> MRRGALPQAPLERTRDFKGSAIRLARRLLPQRALTLAVILLGVGGIAIGVIGPRILGHATDLLFNGVIGRELPAGLTKEQAVEAARARGDGTFADLLSGMDIVPGQGVDFGAVGRTLALALGLYLVAALLVWVQARLLNVTVQRTMVALRAEVQEKIHRLPLSYFDSRQRGEVLSRVTNDVDNIQNSVSMTISQLLTSVLTVFAVLVMML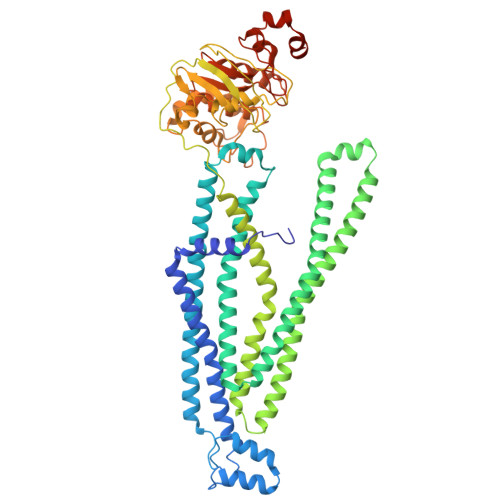TISPLLTLFTVVTVPASLWVTRWITRRSQPLFVAQWRNTGRLAAHLEETYSGFTIVKTFGHREAAAGKFAELNSETQQSSFGAQFFSGLVSPATMFIGNLSYVAVAVVGGLQVATGQITLGSIQAFIQYVRQFNQPLTQVAGMYNTLQSGIASAERVFDLLDTEEESADSPRRADVRTGRVEFEHVSFSYVPGTPVIEDLSLVAEPGSTVAIVGPTGAGKTTLVNLLMRFYDVDSGRITIDGVDIASVSRESLRASIGMVLQDTWLFAGTIYDNIAYGRPDADEDEVIEAATAAYVDRFVHTLPNGYDTRVDDDGGAISAGEKQLITIARAVLARPKLLVLDEATSSVDTRTELLIAHAMAELRRDRTSFIIAHRLSTIRDADLILVMDSGRIIERGTHEELLARHGRYWEMTRVHLGGIKAFHHHHHHHHHH>[8x]MTDPSKLAVAVVCSSNMNRSMEAHNFLAKKGFNVRSYGTGERVKLPGMAFDKPNVYEFGTKYEDIYRDLESKDKEFYTQNGLLHMLDRNRRIKKCPERFQDTKEQFDIIVTVEERVYDLVVM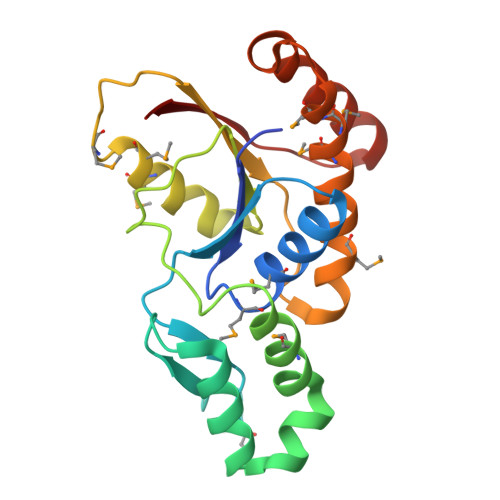HMESMESVDNRPVHVLNVDVVDNAEDALMGAFVITDMINMMAKSTDLDNDIDELIQEFEERRKRVILHSVLFY During transcription of pre-rRNA, the formation of a large knob can be observed by electron microscopy at the 5′ pre-18S portion of the nascent pre-rRNAs. This particle, known as the 90S pre-ribosome or the small subunit (SSU) processome, is responsible for early processing of the 18S rRNA at sites A0, A1 and A2. UTPB is a large complex composed of six proteins Utp1/Pwp2, Utp6, Utp12/Dip2, Utp13, Utp18 and Utp21. Utp1, Utp12, Utp13 and Utp21 all contain two WD domains (WD1 and WD2) followed by 170–260 C-terminal residues that contain no recognizable domain (hereafter called the C-terminal domain, CTD). Utp21 occupies a central position in the UTPB complex as it interacts with all of the other proteins except Utp13.

As part of an effort to understand the structure of UTPB, we have determined the crystal structure of the tandem WD domain of Utp21, the first structure of a UTPB component. The crystal contains one molecule of Utp21, but no Utp18 molecule, in the asymmetric unit. Residues 1–19, 327–337, 393–408 and 660–663 of Utp21 were not modeled due to missing electron density. The tandem WD domains of Utp21 fold into two 7-blade β-propellers, resembling an open clamshell. Blades 1–7 form the N-terminal WD1 domain, and blades 8–14 form the C-terminal WD2 domain. The two β-propellers of Utp21 are more open with an angle of ∼150° compared to those in Aip1 that have an angle of ∼110°. In addition to the core β-propeller domains, Utp21 possesses an extra loop (residues 657–684) following the last strand, 14C. The loop wraps around the side of blades 13 and 14 and inserts into the inter-domain space, making contacts with blade 1. We have found several highly conserved patches on the bottom face of each of the Utp21 WD domains that are potential binding sites for other molecules. In summary, structural mapping of the crosslinking data places the WD domains of Utp1 and Utp18 on two opposite sides of the Utp21 tandem WD domains.

> MSIDLKKRKVEEDVRSRGKNSKIFSPFRIIGNVSNGVPFATGTLGSTFYIVTCVGKTFQIYDANTLHLLFVSEKETPSSIVALSAHFHYVYAAYENKVGIYKRGIEEHLLELETDANVEHLCIFGDYLCASTDDNSIFIYKKSDPQDKYPSEFYTKLTVTEIQGGEIVSLQHLATYLNKLTVVTKSNVLLFNVRTGKLVFTSNEFPDQITTAEPAPVLDIIALGTVTGEVIMFNMRKGKRIRTIKIPQSRISSLSFRTDGSSHLSVGTSSGDLIFYDLDRRSRIHVLKNIHRESYGGVTQATFLNGQPIIVTSGGDNSLKEYVFDPSLSQGSGDVVVQPPRYLRSRGGHSQPPSYIAFADSQSHFMLSASKDRSLWSFSLRKDAQSQEMSQRLHKKQDGGRVGGSTIKSKFPEIVALAIENARIGEWENIITAHKDEKFARTWDMRNKRVGRWTFDTTDDGFVKSVAMSQCGNFGFIGSSNGSITIYNMQSGILRKKYKLHKRAVTGISLDGMNRKMVSCGLDGIVGFYDFNKSTLLGKLKLDAPITAMVYHRSSDLFALALDDLSIVVIDAVTQRVVRQLWGHSNRITAFDFSPEGRWIVSASLDSTIRTWDLPTGGCIDGIIVDNVATNVKFSPNGDLLATTHVTGNGICIWTNRAQFKTVSTRTIDESEFARMALPSTSVR>MPFITVGQENSTSIDLYYEDHGTGTPVVLIHGFPLSGHSWERQSAALLDAGARVITYDRRGFGQSSQPTTGYDYDTFAADLNTVLETLDLQDAVLVGFSMGTGEVARYVSSYGTARIAAVAFLASLEPFLLKTDDNPDGAAPQEFFDGIVAAVKADRYAFYTGFFNDFYNLDENLGTRISEEAVRNSWNTAASGGFFAAAAAPTTWYTDFRADIPRIDVPALILHGTGDRTLPIENTARVFHKALPSAEYVEVEGAPHGLLWTHAEEVNTALLAFLAKAQEAQKQKLLTEVETYVLSIIPSGPLKAEIAQRLEDVFAGKNTDLEVLMEWLKTRPILSPLTKGILGFVFTLTVPSERGLQRRRFVQNALNGNGDPNNMDKAVKLYRKLKREITFHGAKEISLSYSAGALASCMGLIYNRMGAV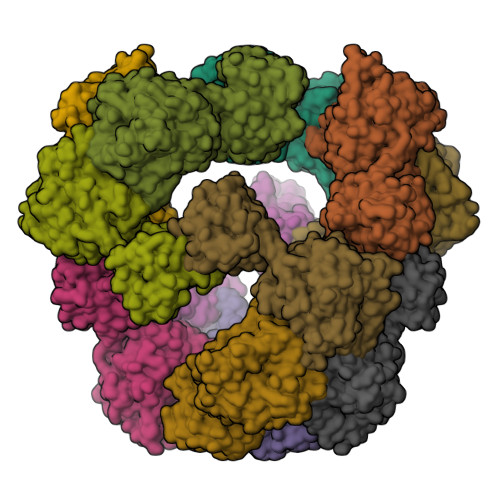TTEVAFGLVCATCEQIADSQHRSHRQLEHHHHHH[6x]> RRRSGSLVYQKRRRRLLPFVSSEDPAQRLKQMGTLASALTELQMEFS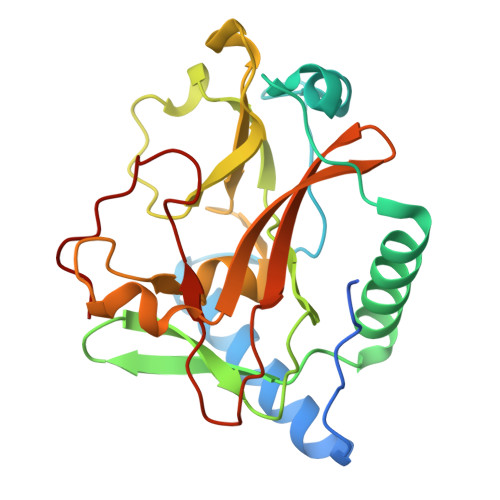DDLTYSSGMAPRSANQARFEEGGMQVLTKEDIETLEQCRAMCKRGDCPPLLVVFDSREGFTVEADGQIKDMTFIAEYTGDVDYIRNREHDDCDSMMTLLLAKDPSSSLVICPDKRGNIARFISGINNHTLDGKKKQNCKCVRYSVNGECRVFLVATRDIAKGERLYYDYNGYEHEYPTQHFV>GAMAKKRGIVQYDFMAESQDELTIKSGDKVYILDDKKSKDWWMCQLVDSGKSGLVPAQ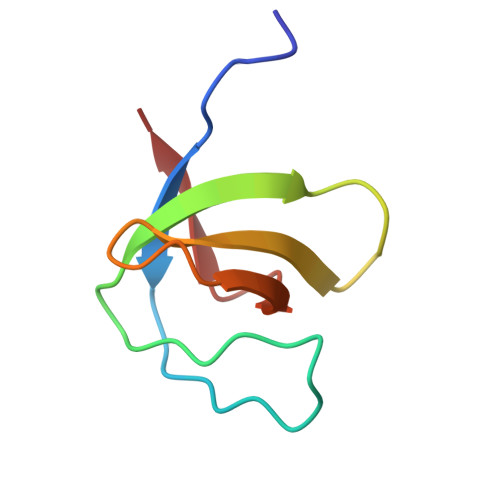FIEPVR[2x]Immature retroviruses are built by the Gag polyprotein; Gag is then cut into domains, and the resulting CA capsid proteins form the mature capsid, which can mediate infection of a new cell. Murine leukemia virus (MLV), the prototypic member of the γ-retroviruses, is commonly used in comparative studies and as a basis for retroviral vector design. The CA domain and immediate downstream residues mediate protein interactions in the immature shell, and, following proteolytic cleavage, CA forms the mature viral capsid. In this study, we have determined the structure of the truncated MLV CA-CTD by X-ray crystallography and have resolved the architecture and CA lattice structures of immature and mature MLV particles by cryo-ET and subtomogram averaging.

No structure of the MLV CA C-terminal domain (CA-CTD) has been determined to date, and the detailed protein interactions in the immature and mature CA lattice of MLV are not known. The structure of the truncated MLV CA-CTD was determined at 1.89-Å resolution by single-wavelength anomalous diffraction (SAD). The crystal belonged to the space group P3121 with one CA-CTDΔCAH dimer in the asymmetric unit. As expected, the overall fold of the MLV CA-CTD is very similar to that observed for other retroviruses (e.g., HIV-1). The dimerization interface includes helix 9, as previously shown for other retroviruses. A short helical turn was found in the MLV CA-CTD between helices 10 and 11 (red) that is not conserved between genera and that contributes to the dimerization interface. We refer to this helix as helix 310b. We compared the arrangement of the monomers in our mature lattice model with the monomer arrangements in the crystal structures of the CA-NTD hexamer and the CA-CTD dimer (present study), respectively. The structures were essentially identical, indicating that the oligomeric forms present in the crystal structures are representative of the arrangement in the mature virus.

>SPTNLAKVKGITQGPNESPSAFLERLKEAYRRYTPYDPEDPGQETNVSMSFIWQSAPDIGRKLERLEDLKSKTLGDLVREAEKIFNK[2x]> MTTYLEFIQQNEERDGVRFSWNVWPSSRLEATRMVVPVAALFTPLKERPDLPPIQYEPVLCSRTTCRAVLNPLCQVDYRAKLWACNFCYQRNQFPPSYAGISELNQPAELLPQFSSIEYVVLRGPQMPLIFLYVVDTCMEDEDLQALKESMQMSLSLLPPTALVGLITFGRMVQVHELGCEGISKSYVFRGTKDLSAKQLQEMLGLSKVPLTQATRGPQVQQPPPSNRFLQPVQKIDMNLTDLLGELQRDPWPVPQGKRPLRSSGVALSIAVGLLECTFPNTGARIMMFIGGPATQGPGMVVGDELKTPIRSWHDIDKDNAKYVKKGTKHFEALANRAATTGHVIDIYACALDQTGLLEMKCCPNLTGGYMVMGDSFNTSLFKQTFQRVFTKDMHGQFKMGFGGTLEIKTSREIKISGAIGPCVSLNSKGPCVSENEIGTGGTCQWKICGLSPTTTLAIYFEVVNQHN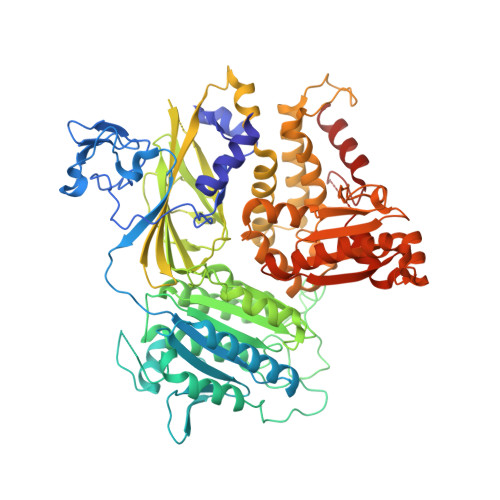APIPQGGRGAIQFVTQYQHSSGQRRIRVTTIARNWADAQTQIQNIAASFDQEAAAILMARLAIYRAETEEGPDVLRWLDRQLIRLCQKFGEYHKDDPSSFRFSETFSLYPQFMFHLRRSSFLQVFNNSPDESSYYRHHFMRQDLTQSLIMIQPILYAYSFSGPPEPVLLDSSSILADRILLMDTFFQILIYHGETIAQWRKSGYQDMPEYENFRHLLQAPVDDAQEILHSRFPMPRYIDTEHGGSQARFLLSKVNPSQTHNNMYAWGQESGAPILTDDVSLQVFMDHLKKLAVSSAA> MEEHTEAGSAPEMGAQKALIDNPADILVIAAYFLLVIGVGLWSMCRTNRGTVGGYFLAGRSMVWWPVGASLFASNIGSGHFVGLAGTGAASGLAVAGFEWNALFVVLLLGWLFAPVYLTAGVITMPQYLRKRFGGRRIRLYLSVLSLFLYIFTKISVDMFSGAVFIQQALGWNIYASVIALLGITMIYTVTGGLAALMYTDTVQTFVILGGACILMGYAFHEVGGYSGLF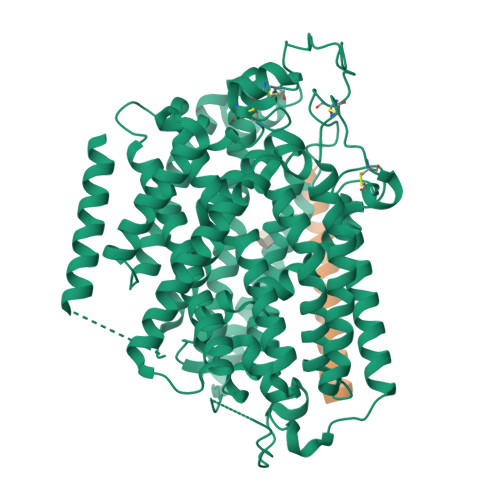DKYLGAATSLTVSEDPAVGNISSFCYRPRPDSYHLLRHPVTGDLPWPALLLGLTIVSGWYWCSDQVIVQRCLAGKSLTHIKAGCILCGYLKLTPMFLMVMPGMISRILYPDEVACVVPEVCRRVCGTEVGCSNIAYPRLVVKLMPNGLRGLMLAVMLAALMSSLASIFNSSSTLFTMDIYTRLRPRAGDRELLLVGRLWVVFIVVVSVAWLPVVQAAQGGQLFDYIQAVSSYLAPPVSAVFVLALFVPRVNEQGAFWGLIGGLLMGLARLIPEFSFGSGSCVQPSACPAFLCGVHYLYFAIVLFFCSGLLTLTVSLCTAPIPRKHLHRLVFSLRHSKEEREDLDADEQQGSSLPVQNGCPESAMEMNEPQAPAPSLFRQCLLWFCGMSRGGVGSPPPLTQEEAAAAARRLEDISEDPSWARVVNLNALLMMAVAVFLWGFYA;> MSALSLLILGLLTAVPPASCQQGLGNLQPWMQGLIAVAVFLVLVAIAFAVNHFWCQEEPEPAHMILTVGNKADGVLVGTDGRYSSMAASFRSSEHENAYENVPEEEGKVRSTPM>PKQVGNAQHLYDNYDLVPAMIAEVNPRDMVVMALVNTNVDPTLPPRWALATRNITAIPGIEGDTRKVGTRIPAVAVTGQRSVGNQDSWDQISPMPIAWATPDSSVIARAESTIPSEQWTTLSKNLNKLD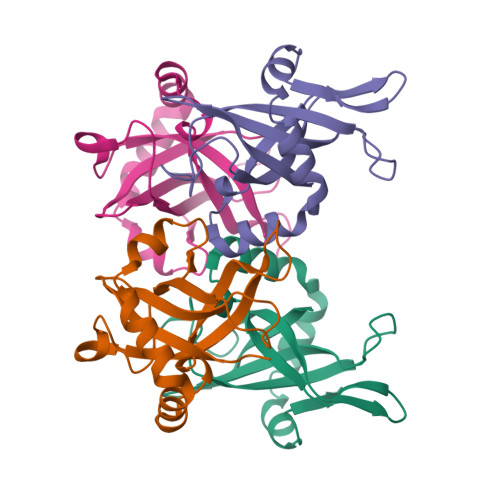QVRETKFDLLEL[2x]> MENTENSVDSKSIKNLEPKIIHGSESMDSGISLDNSYKMDYPEMGLCIIINNKNFHKSTGMTSRSGTDVDAANLRETFRNLKYEVRNKNDLTREEIVELMRDVSKEDHSKRSSFVCVLLSHGEEGIIFGTNGPVDLKKITNFFRGDRCRALTGKPKLFI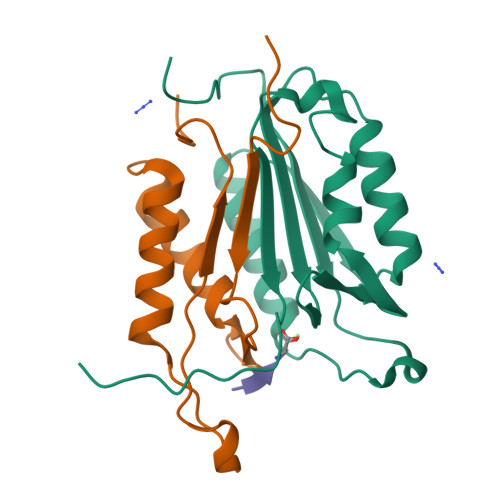IQACRGTELDCGIETD;> SGVDDDMACHKIPVEADFLYAYSTAPGYYSWRNSKDGSWFIQSLCAMLKQYADKLEFMHILTRVNRKVATEFESFSFDATFHAKKQIPCIVSMLTKELYFYH> MGSHHHHHHSQDPMAYSTREILLALCIRDSRVHGNGTLHPVLELAARETPLRLSPEDTVVLRYHVLLEEIIERNSETFTETWNRFITHTEHVDLDFNSVFLEIFHRGDPSLGRALAWMAWCMHACRTLCCNQSTPYYVVDLSVRGMLEASEGLDGWIHQQGGWSTLIEDNIPG;> EEQWAREIGAQLRRMA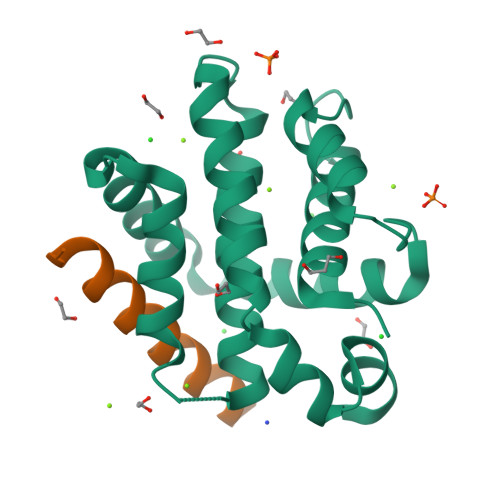DDLNAQYERR>[2x]HHHHHHGSMGYPVIVEATRSPIGKRNGWLSGLHATELLGAVQKAVVDKAGIQSGLHAGDVEQVIGGCVTQFGEQSNNISRVAWLTAG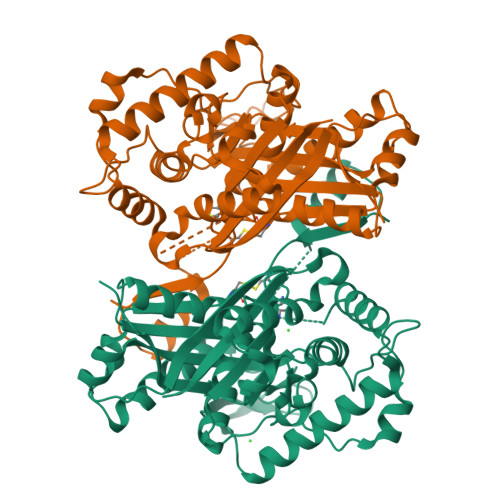LPEHVGATTVDCQCGSGQQANHLIAGLIAAGAIDVGIACGIEAMSRVGLGANAGPDRSLIRAQSWDIDLPNQFEAAERIAKRRGITREDVDVFGLESQRRAQRAWAEGRFDREISPIQAPVLDEQNQPTGERRLVFRDQGLRETTMAGLGELKPVLEGGIHTAGTSSQISDGAAAVLWMDEAVARAHGLTPRARIVAQALVGAEPYYHLDGPVQSTAKVLEKAGMKIGDIDIVEINEAFASVVLSWARVHEPDMDRVNVNGGAIALGHPVGCTGSRLITTALHELERTDQSLALITMCAGGALSTGTIIERI>MTDAVAGKTSLPPPVAIIVGHNIDASAMPLTYERNRFVIDMLQHYACPVFSHKKSGDAMNTVSSDVFEWVLEPFPVVGVEDMTAFHDRAYLNYLSIREALSEVDERASTVKPPLRVLPDLVPIPADEEYGLVNENMPFVGMWRTIQATVSGTLLAARLLAQPGRFAAIHWFGGRHHAKKSTAGGFCFANDVVLGVLELKKLLSSDKNGILVVDVDAHHGDGTQSAFLHDNSVLTLSMHAHGVGIFPGTGGIEEIGAGLGRGFTMNVPLPEGATDILAVTLMYRSIHFAFKKLGEGLAAIVIVCGSDALSGDPLGALNLTVGGMQSIIRLLLKEAARRSLKVLLLGAGGYVDTSCARLAGVVTKDVLSCAAAMRLGKTEYFGDSANLGDNLGVAVPEGCEYFTRYGPSFLMHGLPPARVSKLYRLPYGSPLFMRMQRAATKEALRRRLN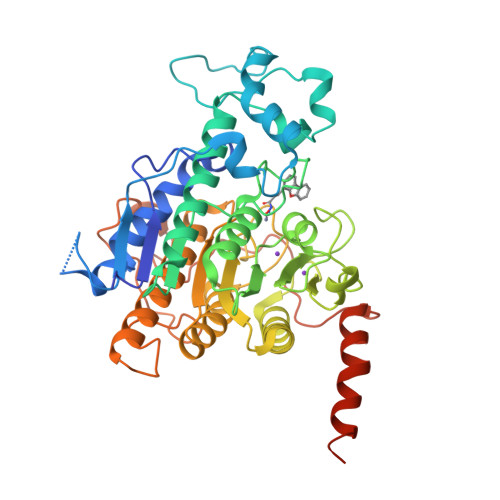QEQDEEEDAEDSGLEVLFQ[2x]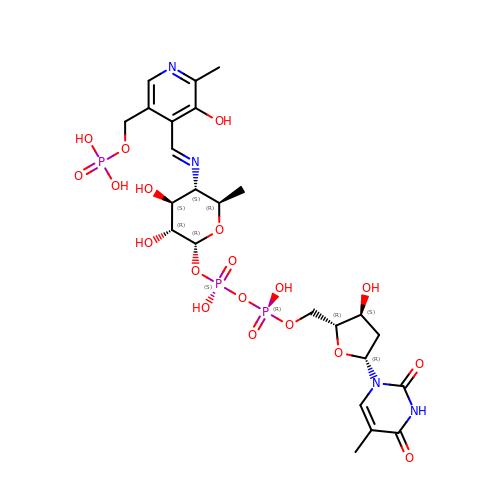(2R,3R,4S,5S,6R)-3,4-DIHYDROXY-5-[({3-HYDROXY-2-METHYL-5-[(PHOSPHONOOXY)METHYL]PYRIDIN-4-YL}METHYL)IMINO]-6-METHYLTETRAHYDRO-2H-PYRAN-2-YL [(2R,3S,5R)-3-HYDROXY-5-(5-METHYL-2,4-DIOXO-3,4-DIHYDROPYRIMIDIN-1(2H)-YL)TETRAHYDROFURAN-2-YL]METHYL DIHYDROGEN DIPHOSPHATE | C24 H35 N4 O19 P3 | LEIRFGMKEVPNBT-ZBVJAJKCSA-N>[2x]SHVDPRIQGELEKLNQSTDDINRRETELEDARQKFRSVLVEATVKLDELVKKIGKAVEDSKPYWEARRVARQAQLEAQKATQDFQRATEVLRAAKETISLAEQRLLED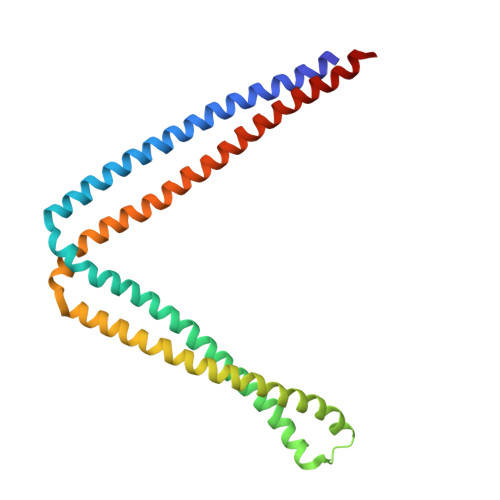DKRQFDSAWQEMLNHATQRVMEAEQTKTRSELVHKETAARYNAAMGRMRQLEKKLKRAINKSKPYFELKAKYYVQLEQLKKTVDDLQAKLTLAKGEYKMALKNLEMISDEIHEAAASSAM>[2x]MFKKWKKFGISSLAL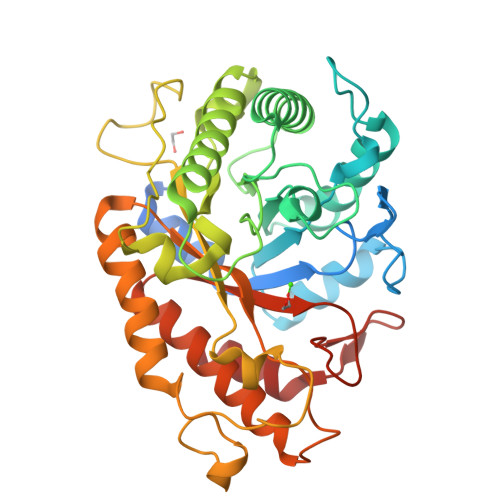VLVAAVAFTGWSAKASAADASQIVSEMGAGWNLGNQLEAAVNGTPNETAWGNPTVTPELIKKVKAAGFKSIRIPVSYLNNIGSAPNYTINAAWLNRIQQVVDYAYNEGLYVIINIHGDGYNSVQGGWLLVNGGNQTAIKEKYKKVWQQIATKFSNYNDRLIFESMNEVFDGNYGNPNSAYYTNLNAYNQIFVDTVRQTGGNNNARWLLVPGWNTNIDYTVGNYGFTLPTDNYRSSAIPSSQKRIMISAHYYSPWDFAGEENGNITQWGATSTNPAKKSTWGQEDYLESQFKSMYDKFVTQGYPVVIGEFGSIDKTSYDSSNNVYRAAYAKAVTAKAKKYKMVPVYWDNGHNGQHGFALFNRSNNTVTQQNIINAIMQGMQ> SVSSIVSRAQFDRMLLHRNDGACQAKGFYTYDAFVAAAAAFPGFGTTGSADAQKREVAAFLAQTSHETTGGWATAPDGAFAWGYCFKQERGASSDYCTPSAQWPCAPGKRYYGRGPIQLSHNYNYGPAGRAIGVDLLANPDLVATDATVGF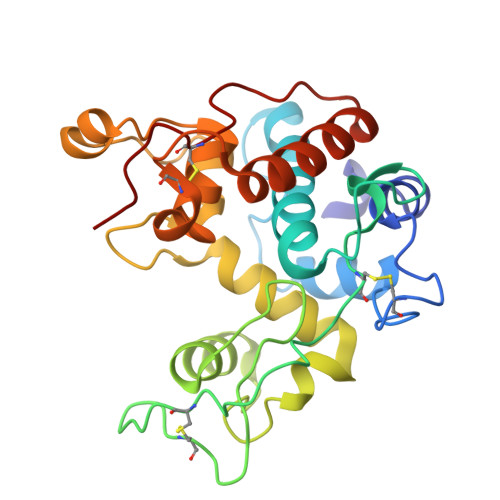KTAIWFWMTAQPPKPSSHAVIAGQWSPSGADRAAGRVPGFGVITNIINGGIECGHGQDSRVADRIGFYKRYCDILGVGYGNNLDCYSQRPFA> GPGSRIAEEAVGNVSTGALRTITLSKMKQSLGISISGGIESKVQPMVKIEKIFPGGAAFLCGDLQAGFELVAVDGESLEQVTHQRAV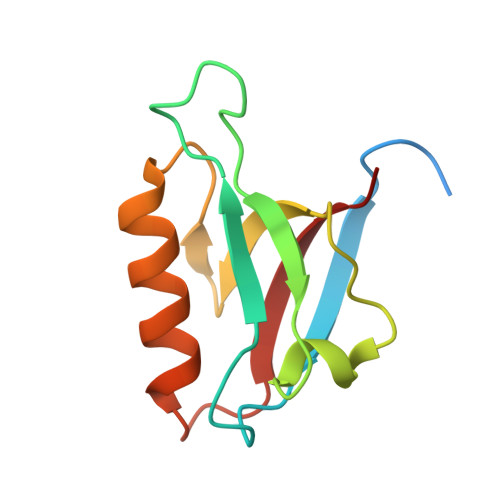DTIRRAYRNKAREPMELVVRVP5-(7-(5-HYDRO-4-ETHYL-2-OXAZOLYL)PHENOXY)HEPTYL)-3-METHYL 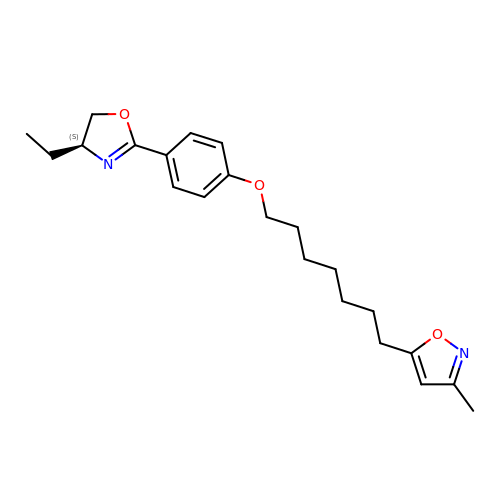ISOXAZOLE | C22 H30 N2 O3 | PZDSRPCFNWOUFP-IBGZPJMESA-N Serine O-acetyltransferase (CysE) is an enzyme in many bacteria that catalyzes the first step in l-cysteine biosynthesis by transferring an acetyl group from acetyl coenzyme A (acetyl-CoA) to l-serine to form O-acetylserine. Lack of the CysE/CysK-dependent l-cysteine biosynthesis pathway in mammals suggests that those bacterial enzymes may become targets for antimicrobial agents. In this study, we used recombinant CysE cloned from Salmonella Typhimurium (StCysE). Here, we demonstrated that alkyl gallates such as octyl gallate (OGA) could act as potent CysE inhibitors in vitro and in bacteria.

In the first step, l-serine is converted to O-acetylserine (OAS), with acetyl coenzyme A (acetyl-CoA) used as a co-substrate, by means of the catalytic action of serine O-acetyltransferase (CysE).

>MHHHHHHDPPCEELEIVWKNIKAEARALADCEPMLASFYHATLLKHENLGSALSYMLANKLASPIMPAIAIREVVEEAYAADPEMIASAACDIQAVRTRDPAVDKYSTPLLYLKGFHALQAYRIGHWLWNKGRRALAIFLQNQVSVSFQVDIHPAAKIGRGIMLDHATGIVVGETAVIEDDVSILQSVTLGGTGKTSGDRHPKIREGVMIGAGAKILGNIEVGRGAKIGAGSVVLQPVPPHTTAAGVPARIVGKPGSDKPSMDMDQHFNGIHHTFEYGDG[3x]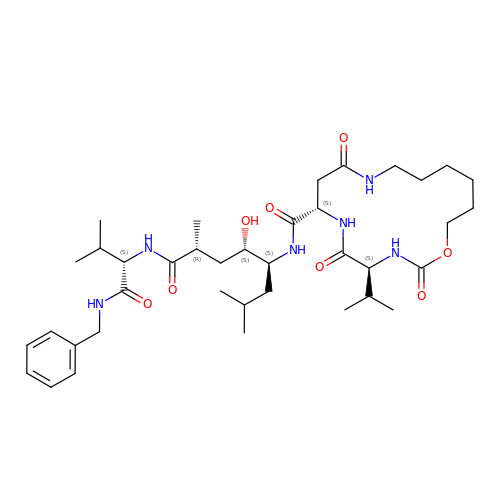N-[(4S,5S,7R)-8-({(S)-1-[(BENZYLAMINO)OXOMETHYL]-2-METHYLPROPYL}AMINO)-5-HYDROXY-2,7-DIMETHYL-8-OXO-OCT-4-YL]-(4S,7S)-4-ISOPROPYL-2,5,9-TRIOXO-1-OXA-3,6,10-TRIAZACYCLOHEXADECANE-7-CARBOXAMIDE | C38 H62 N6 O8 | QJAPFAZHNSZLJE-CWURXVSKSA-N> MGSSHHHHHHSQDPAEKQKHDGRVKIGHYVLGDTLGVGTFGKVKIGEHQLTGHKVAVKILNRQKIRSLDVVGKIKREIQNLKLFRHPHIIKLYQVISTPTDFFMVMEYVSGGELFDYICKHGRVEEMEARRLFQQILSAVDYCHRHMVVHRDLKPENVLLDAHM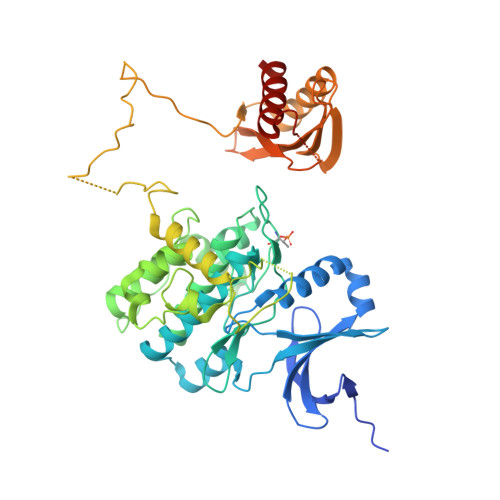NAKIADFGLSNMMSDGEFLRTSCGSPNYAAPEVISGRLYAGPEVDIWSCGVILYALLCGTLPFDDEHVPTLFKKIRGGVFYIPEYLNRSVATLLMHMLQVDPLKRATIKDIREHEWFKQGLPSYLFPEDPSYDANVIDDEAVKEVCEKFECTESEVMNSLYSGDPQDQLAVAYHLIIDNRRIMNQASEFYLASSPPSGSFMDDSAMHIPPGLKPHPERMPPLIADSPKARCPLDALNTTKPKSLAVKKAKWHLGIRSQSKPYDIMAEVYRAMKQLDFEWKVVNAYHLRVRRKNPVTGNYVKMSLQLYLVDNRSYLLDFKSIDDEVVEQRSGSSTPQRSCSAAGLHRPRSSFDSTTAESHSLSGSLTGSLTGSTLSSVSPRLGSHTMDFFEMCASLITTLAR N-{4-[(2,2-dimethylpropyl)carbamamido]phenyl}-1H-indazole-7-carboxamide 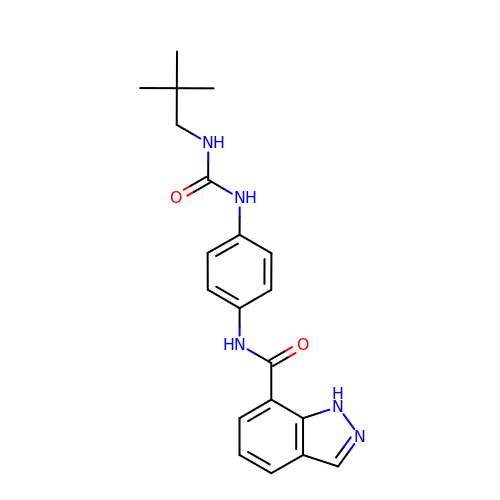| C20 H23 N5 O2 | RKYDKVAEPCHCFH-UHFFFAOYSA-N In order to understand the structural basis for the effect of N6‐methyladenine on k‐turn conformation, we have used X‐ray crystallography to investigate the structural effect of this modification on different base pairs involving adenine. Each species was formed by the hybridization of a self‐complementary strand that contains a 5‐bromocytosine nucleotide used to calculate phases for the diffraction in most cases. Crystallography reveals that N6‐methylation of adenine prevents the formation of trans Hoogsteen‐sugar A·G base pairs, explaining why the box C/D RNA cannot adopt its kinked conformation. More generally, our data indicate that sheared A·G base pairs (but not Watson–Crick base pairs) are more susceptible to disruption by N6mA methylation and are therefore possible regulatory sites.

We synthesized a second self‐complementary RNA strand that would hybridize to form central consecutive G·A pairs flanked by G‐C base pairs, with and without a methyl group on the adenine N6. The two species adopted closely similar structures, with the G·A and G·6mA forming cis Watson–Crick base pairs in both cases that are well superimposed, irrespective of the presence of the methyl group on AN6. In both structures, the G·A base pairs are cis Watson–Crick pairs connected by two hydrogen bonds. We conclude that N6‐methylation of adenine need not lead to disruption of the Watson–Crick G·A pairs.

>GCCGGACGGC[2x]>MIAYHTLTKALLFPDIDQYQHWHHVAPMLAKMLVDGKYSIHQQYEYLCLFAQLVAPVLGPYPSPGRDVYRCTLGGNMTVELSQNFQRSGSTTRIAFEPVRYQASVGHDRFNRTSVNAFFSQLQLLVKSVNIELHHLLSEHLTLTAKDERNLNEEQLTKYLTNFQVKTQYVVALDLRKTGIVAKEYFFPGIKCAATGQTGSNACFGAIRAVDKDGHLDSLCQLIEAHFQQSKIDDAFLCCDLVDPAHTRFKVYIADPLVTLARAEEHWTLGGRLTDEDAAVGLEIIRGLWSELGIIQGPLEPSAMMEKGLLPIMLNYEMKAGQRLPKPKLYMPLTGIPETKIARIMTAF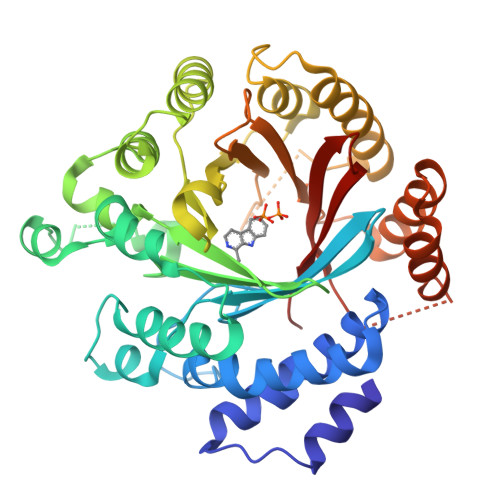FQRHDMPEQAEVFMENLQAYYEGKNLEEATRYQAWLSFAYTKEKGPYLSIYYFWPE[4x]> MCYASMEMSAPIRFGTEGFRGVIAREFTFATLHRLAEAYGRHLLERGGGLVVVGHDTRFLADAFARALSGHLAGMGLKVVLLKGPVPTPLLSFAVRHLKAAGGAMLTASHNPPQYLGVKFKDATGGPIAQEEAKAIEALVPEEARALEGAYETLDLREAYFEALKAHLDLKALSGFSGVLYHDSMGGAGAGFLKGFLRHVGLEIPVRPIREEPHPLFHGVNPEPIPKNLGVTLAVLGPETPPSFAVATDGDADRVGVVLPGGVFFNPHQVLTTLALYRFRKGHRGRAVKNFAVTWLLDRLGERLGFGVTTTPVGFKWIKEEFLKGDCFIGGEESGGVGYPEHLPERDGILTSLLLLESVAATGKDLAEQFKEV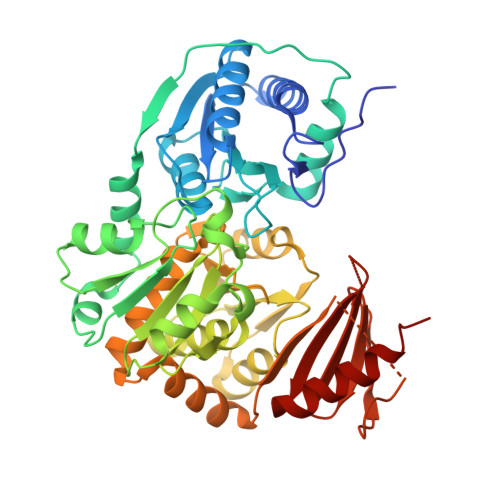EALTGLTHAYDRLDLPLKAPLDLTPFREPRPLAGLTPKGVDTLDGVKWLYEEAWVLFRASGTEPVVRIYVEAQSPELVRALLEEARKLVEG>[8x]MTRAINDPGNEDPGSLLETDADALLGGAAAQAPEERCRLAAQACIRACERYLALCTESSREQRQHAGDCADLCRLAALLLERRSPWAPAACELAARYALAC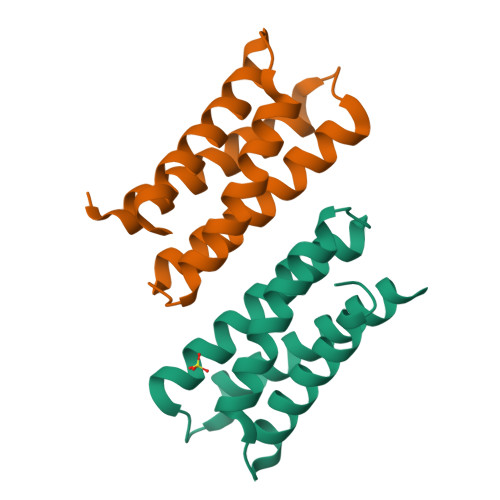AERCDGDEPLERECAGACRRFVEACRPLLPALEHHHHHH>[2x]QKYNPFRYVELFIVVDQGMVTKNNGDLDKIKA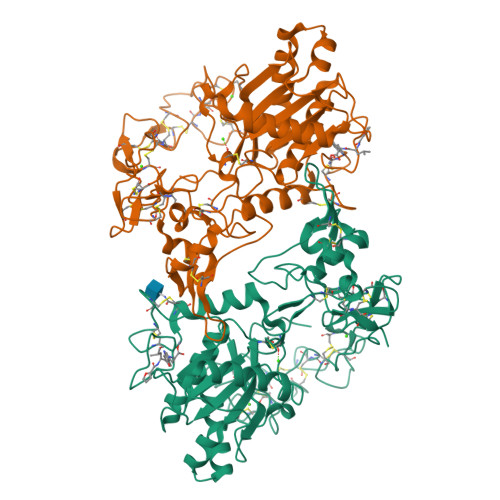RMYELANIVNEILRYLYMHAALVGLEIWSNGDKITVKPDVDYTLNSFAEWRKTDLLTRKKHDNAQLLTAIDFNGPTIGYAYIGSMCHPKRSVAIVEDYSPINLVVAVIMAHEMGHNLGIHHDTDFCSCGDYPCIMGPTISNEPSKFFSNCSYIQCWDFIMKENPQCILNEPLGTDIVSPPVCGNELLEVGEECDCGTPENCQNECCDAATCKLKSGSQCGHGDCCEQCKFSKSGTECRASMSECDPAEHCTGQSSECPADVFHKNGQPCLDNYGYCYNGNCPIMYHQCYALFGADVYEAEDSCFKDNQKGNYYGYCRKENGKKIPCAPEDVKCGRLYCKDNSPGQNNPCKMFYSNDDEHKGMVLPGTKCADGKVCSNGHCVDVATAY[(1R)-1-chloroethyl]benzene | 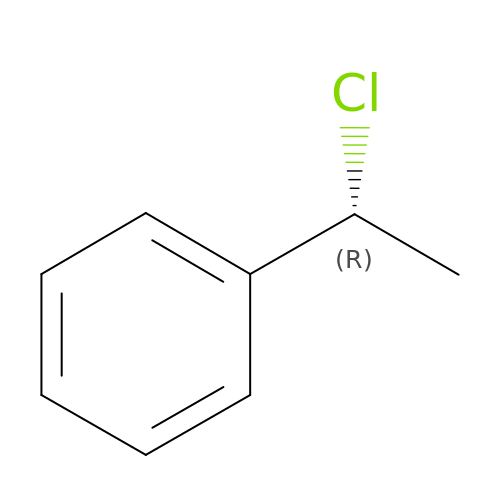C8 H9 Cl | GTLWADFFABIGAE-SSDOTTSWSA-N> MTAIAPVITIDGPSGAGKGTLCKAMAEALQWHLLDSGAIYRVLALAALHHHVDVASEDALVPLASHLDVRFVSTNGNLEVILEGEDVSGEIRTQEVANAASQVAAFPRVREALLRRQRAFRELPGLIADGRDMGTVVFPDAPVKIFLDASSEERAHRRMLQLQEKGFSVNFERLLAE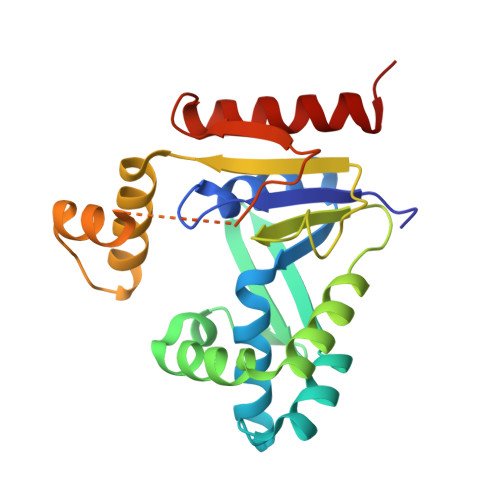IKERDDRDRNMAVAPLVPAADALVLDSTTLSIEQVIEKALQYARQKLALA> GPKLLMIIHDRREFAKFEK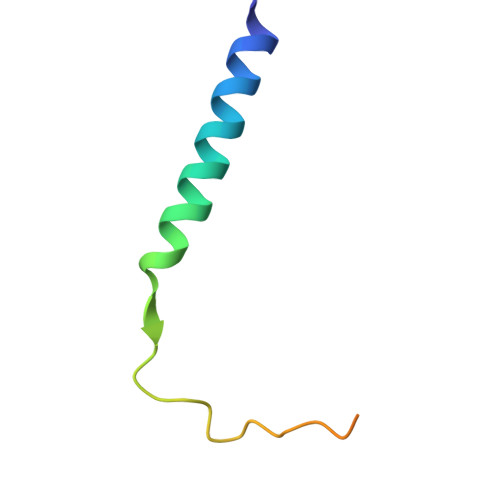EKMNAKWDTQENPIYKSPINNFKNPNYGRKAGL> KNTQTLMPLTERVNVQADSARINQIIDGCWVAVGTNKPHAIQRDFTNLFDGKPSYRFELKTEDNTLEGYAKGETKGRAEFSYCYATSDDFRGLPADVYQKAQITKTVYHHGKGACPQGSSRDYEFSVYIPSSLDSNVSTIFAQWHGMPDRTLV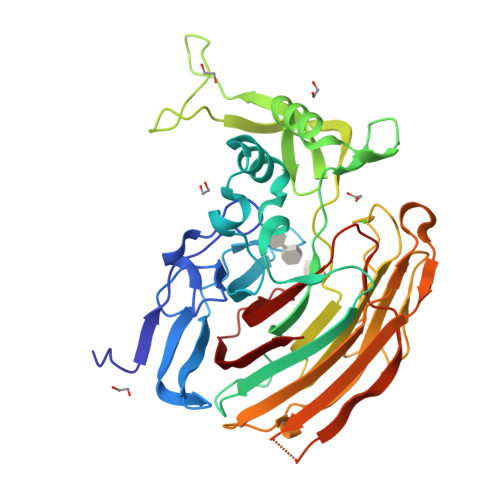QTPQGEVKKLTVDEFVELEKTTFFKKNVGHEKVARLDKQGNPVKDKNGKPVYKAGKPNGWLVEQGGYPPLAFGFSGGLFYIKANSDRKWLTDKDDRCNANPGKTPVMKPLTSEYKASTIAYKLPFADFPKDCWITFRVHIDWTVYGKEAETIVKPGMLDVRMDYQEQGKKVSKHIVDNEKILIGRNDEDGYYFKFGIYRVGDSTVPVCYNLAGYSER>[4x]GTQGFAVL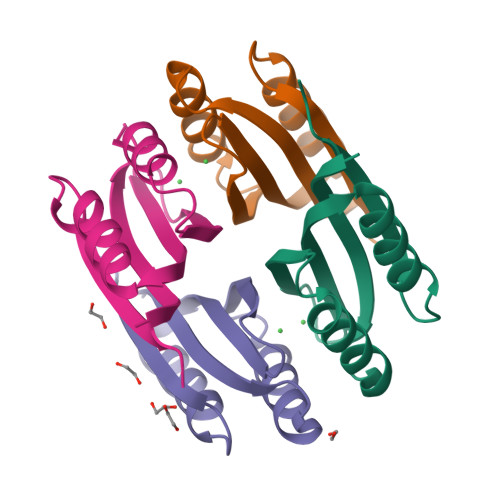SYVYEHEKRDLASRIVSTQHHHHDLSVATLHVHINHDDCLEIAVLKGDMGDVQHFADDVIAQRGVRHGHLQCLPKED>MGDPEEYEDQLEETLEQKEYEDHDSVSIPMEEAEGDTIQEEEAEARVNQLTDTDYHTTSQHPETHKVCVQLRELVMDEKNQEIQWMETARWVGLEENLGKDGIWGRPHLPYLNFWSLLELQKAFAKGTVLLDLPGKSLAEVANQLLDRFTFEGQIQPDDQDNLLRVLLLKHSHASDMEALGGVKPVVVTHSGDPSEPLLPQHPSLETELFCEQGEGSTRGHAPEILGKSPQDWEATLVLVGCARFLKRPVLGFVRLKEPMEPEPKPEGSEEPAVPVRFLIVLLGPEGPNINYTQLGRAAATLMSERVFWNDAYLAQSKETLVQSLEGFLDCSLVLPPLDAPSEKALLSLVPVQKELLRRRYLPSPAKPDPSIFKDLDVKKGPGDTPEDPLQRTGKLFGGLVRDIRRRYPRYLSDITDALSPQVLSAIIFIYFAALTPAITFGGLLGDKTENMIGVSELLLSTALQGIIFSLLGAQPLLVLGFSGPLLVFEEAFYSFCQTNNLEYIVGRVWIGFWLILLVVLVVAFEGSFLVRFISRYTQEIFSFLISLIFIYETFYKLVTIFQDHPLQKNYDHDVLTTPKPQAALPNTALLSLVLMAGTFFLAMMLRKFKNSSYFPGKLRRIIGDFGVPISILIMVMVDALIQDTYTQKLSVPEGLSVSNPTERDWLIHPLGIRVEFPIWMMFASALPAL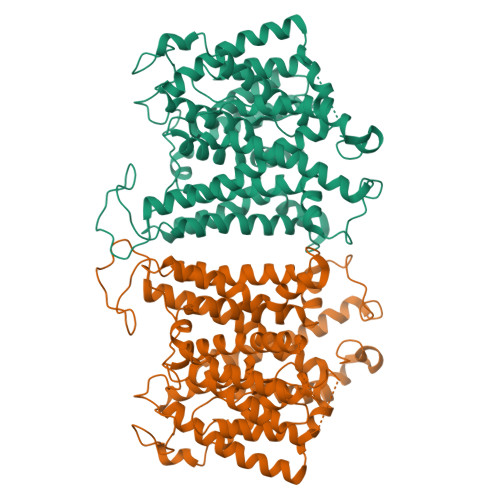LVFILIFLESQITTLIISKPERKMVKGSGFHLDLLLIIGMGGVGAIFGMPWLSATTVRTVTHANALTVMSKDSTPGAVSQIQGVKEQRISGLLVAVLVGVSILMGPVLRHIPLAVLFGIFLYMGVTSLSGIQLFDRVLLLLKPRKYYPEVPYARRVKTWRMHLFTITQIVCLVVLWVVRSIKQISLALPFILILTVPLRRFLLPFIFRDMELKLLDADDVKLNLDEQNGQDEYDEVAMPV[2x]> ASMQKLINSVQNYAWGSKTALTELYGIANPQQQPMAELWMGAHPK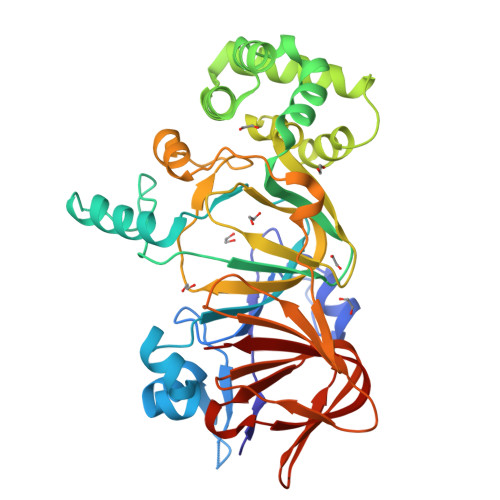SSSRITTANGETVSLRDAIEKNKTAMLGEAVANRFGELPFLFKVLCAAQPLSIQVAPNKRNSEIGFAKENAAGIPMDAAERNYKDPNHKPELVFALTPFLAMNAFREFSDIVSLLQPVAGAHSAIAHFLQVPNAERLSQLFASLLNMQGEEKSRALAVLKAALNSQQGEPWQTIRVISEYYPDDSGLFSPLLLNVVKLNPGEAMFLFAETPHAYLQGVALEVMANSDNVLRAGLTPKYIDIPELVANVKFEPKPAGELLTAPVKSGAELDFPIPVDDFAFSLHDLALQETSIGQHSAAILFCVEGEAVLRKDEQRLVLKPGESAFIGADESPVNASGTGRLARVYNKL>[2x]MHHHHHHAAGIPMNNPAIKRIGNHITKSPEDKREYRGLELANGIKVLLISDPTTDKSSAALDVHIGSLSDPPNIAGLSHFLQHMLFLGTKKYPKENEYSQFLSEHAGSSNAFTSGEHTNYYFDVSHEHLEGALDRFAQFFLSPLFDESAKDREVNAVDSEHEKNVMNDAWRLFQLEKATGNPKHPFSKFGTGNKYTLETRPNQEGIDVRQELLKFHSAYYSSNLMAVVVLGRESLDDLTNLVVKLFSEVENKNVPLPEFPEHPFQEEHLKQLYKIVPIKDIRNLYVTFPIPDLQKYYKSNPGHYLGHLIGHEGPGSLLSELKSKGWVNTLVGGQKEGARGFMFFIINVDLTEEGLLHVEDIILHMFQYIQKLRAEGPQEWVFQELKDLNAVAFRFKDKERPRGYTSKIAGILHYYPLEEVLTAEYLLEEFRPDLIEMVLDKLRPENVRVAIVSKSFEGKTDRTEEWYGTQYKQEAIPDEVIKKWQNADLNGKFKLPTKNEFIPTNFEILPLEKEATPYPALIKDTAMSKLWFKQDDKFFLPKANLNFEFFSPFAYVDPLHSNMAYLYLELLKDSLNEYAYAAELAGLSYDLQNTIYGMYLSVKGYNDKQPILLKKIIEKMATFEIDEKRFEIIKEAYMRSLNNFRAEQPHQHAMYYLRLLMTEVAWTKDELKEALDDVTLPRLKAFIPQLLSRLHIEALLHGNITKQAALGIMQMVEDTLIEHAHTKPLLPSQLVRYREVQLPDRGWFVYQQRNEVHNNSGIEIYYQTDMQSTSENMFLELFAQIISEPAFNTLRTKEQLGYIVFSGPRRANGIQGLRFIIQSEKPPHYLESRVEAFLITMEKSIEDMTEEAFQKHIQALAIRRLDKPKKLSAESAKYWGEIISQQYNFDRDNTEVAYLKTLTKEDIIKFYKEMLAVDAPRRHKVSVHVLAREMDSNPVVGEFPAQNDINLSQAPALPQPEVIQNMTEFKRGLPLFPLVKPHINFMAAKL;>APMGSDPPTACCFSYTARKLPRNFVVDYYETSSLCSQPAVVFQTKRSKQVCADPSESWVQEYVYDLELN[2x]

CC chemokine ligands (CCL) comprise 8-14 kDa chemotactic cytokines (chemokines) involved in diverse immune functions. Extensive structural analyses reveal that most chemokines share a common core structure: an N-terminal extension followed by a 310 helical turn, an anti-parallel three-stranded β-sheet, and an α-helix. CC chemokines also readily dimerize, primarily through the formation of an anti-parallel β-sheet at their N-termini. Certain chemokines, e.g. CCL3, CCL4, and CCL5 form polydisperse, high MW reversible polymers in excess of 600 kDa without the assistance of GAG.

Insulin degrading enzyme (IDE) is a M16 zinc-metalloprotease that selectively degrades amyloidogenic peptides such as amyloid β, peptide vital for the progression of Alzheimer’s disease. To understand the molecular basis of CCL4 recognition by IDE, we solved the structure of CCL4 bound human IDE at 3.2Å. In order to avoid cleavage of CCL4, E111Q was introduced to IDE to remove the catalytic base required for the protonation of a catalytic water. The overall fold of the complex shows that, as in previously reported structures of substrate-bound IDE, IDE adopts a closed conformation. We only could model three N terminal residues of CCL4 at the exosite of IDE and 6 residues of CCL4 at the catalytic cleft of IDE. At the exosite, the electron density corresponds to three N-terminal residues of CCL4, which form hydrogen bonds with the E341 carboxyl, and G361 and L359 carbonyl groups of IDE. At the catalytic site, aa 42-47 of CCL4 are clearly visible. We find that Q111 is in close proximity to the scissile bond of a major cleavage site, K45-R46, with the proper geometry for the proteolytic reaction. In comparison with CCL4 NMR structures, our structure of CCL4-bound IDE reveals that, in order to bind the catalytic chamber of IDE, both the N-terminus and the cleavage loop region of CCL4 must undergo a substantial conformational change upon their interaction with IDE. Most noticeably, the α-helical region of residues 42-47 needs to transform into a β-strand to extend a β-sheet into the catalytic cleft of IDE.(4~{S})-4-(4-chlorophenyl)-5-[(1~{S})-1-(3-chlorophenyl)ethyl]-2-(2,4-dimethoxypyrimidin-5-yl)-3-propan-2-yl-4~{H}-pyrrolo[3,4-d]imidazol-6-one 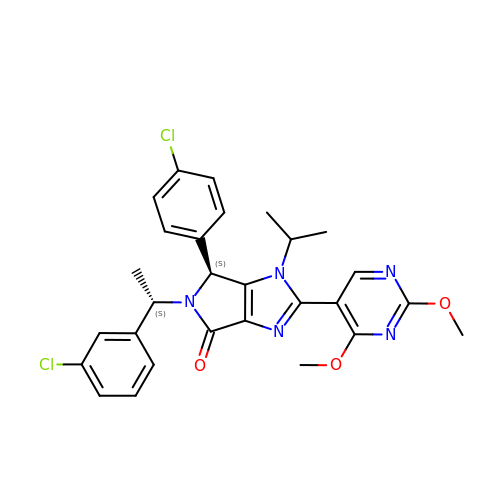| C28 H27 Cl2 N5 O3 | PYBJKPRTJDONOS-HJPURHCSSA-N4-(morpholin-4-yl)-6-[4-(trifluoromethyl)phenyl]pyrimidin-2-amine | C15 H15 F3 N4 O | 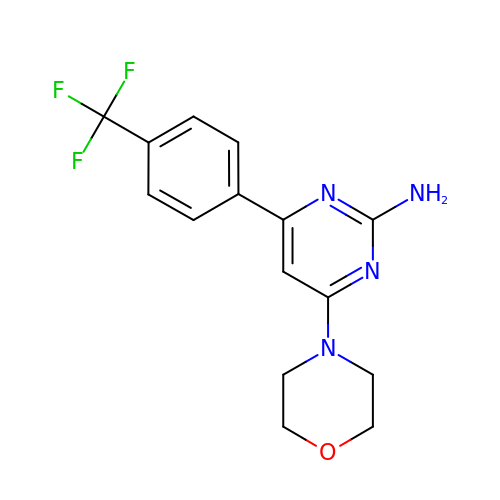XZLXJMNYYMKDDT-UHFFFAOYSA-N> MRGSHHHHHHGMASMSVSTASTEMSVRKIAAHMKSNPNAKVIFMVGAGISTSCGIPDFRSPGTGLYHNLARL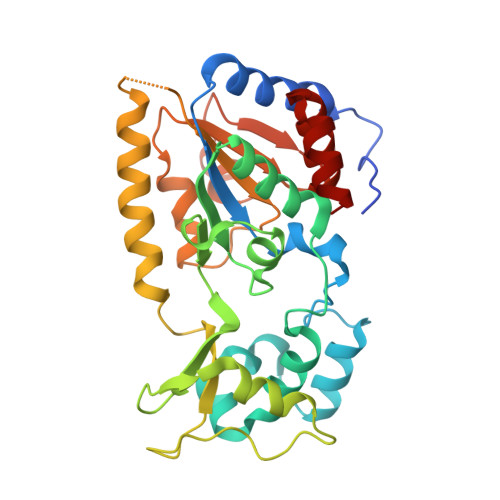KLPYPEAVFDVDFFQSDPLPFYTLAKELYPGNFRPSKFHYLLKLFQDKDVLKRVYTQNFDTLERQAGVKDDLIIEAHGSFAHCHCIGCGKVYPPQVFKSKLAEHPIKDFVKCDVCGELVKPAIVFFGEDLPDSFSETWLNDSEWLREKITTSGKHPQQPLVIVVGTSLAVYPFASLPEEIPRKVKRVLCNLETVGDFKANKRPTDLIVHQYSDEFAEQLVEELGWQEDFEKILTAQ>[3x]MLDEKSSNTAVVVVLCTAPDEATAQDLAAKVLAEKLAACATLIPGATSLYYWE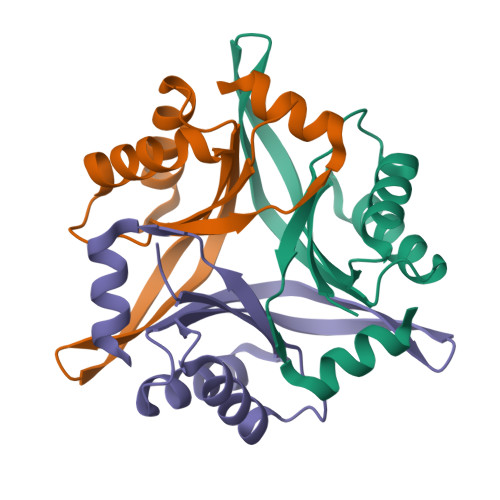GKLEQEYVVQMILKTTVSHQQALLECLKSHHPYQTPELLVLPVTHGDTDYLSWLNASLR> SGISLDNSYKMDYPEMGLCIIINNKNFHKSTGMTSRSGTDVDAANLRETFRNLKYEVRNKNDLTREEIVELMRDVSKEDHSKRSSFVCVLLSHGEEGIIFGTNGPVDLKKITNFFRGDRCRSLTGKPKLFIIQACRGTELDCGIETDSGVDDDMACHKI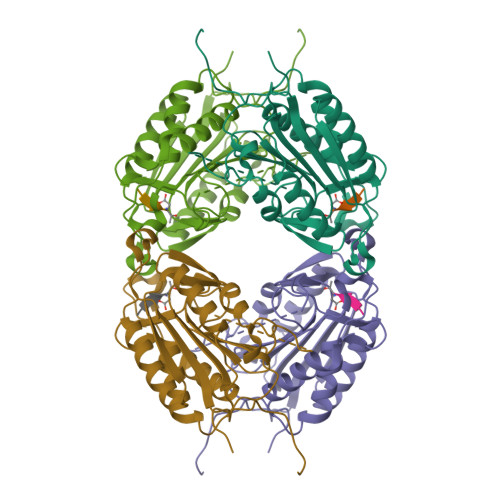PVEADFLYAYSTAPGFYSWRNSKDGSWFIQSLCAMLKQYADKLEFMHILTRVNRKVATEFESFSFDATFHAKKQIPCIVSMLTKELYFYHH AZELAIC ACID | C9 H16 O4 | 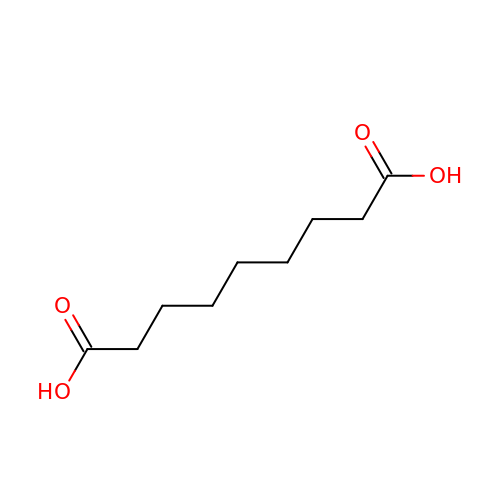BDJRBEYXGGNYIS-UHFFFAOYSA-N> ANENILKLKLYRSLGVILDLENDQVLINRKNDGNIDILPLDNNLSDF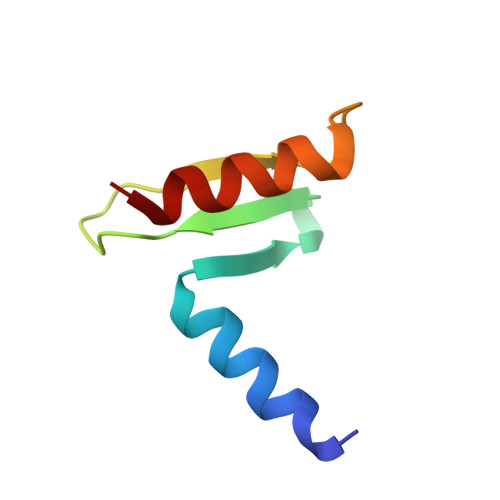YKTKYIWERLGK Proteins of the Ras superfamily of small GTPases regulate a variety of cellular processes such as intracellular transport, cell shape and motility, as well as differentiation and growth. For all of these processes, switching between the active GTP-bound and the inactive GDP-bound states is of fundamental importance. We describe here the synthesis of reactive acryl derivatives of guanine nucleotides that are able to react covalently with strategically placed cysteines in GTPases to lock them into their functional states in an irreversible manner. Extensive analysis of biochemical and structural features demonstrate the maintenance of the signalling ability of the modified GTPases.

Extending the labelling experiments to other GTPases, placing a cysteine at the position equivalent to E35 in Rab1b led to covalent interaction with aGTP for all those tested (Rab5A, Rab6A, Rab7A, Rab8A, Ypt7, HRas and Cdc42), albeit at variable rates, but substitution of cysteine at positions corresponding to L125 in Rab1b only led to covalent reaction in the case of Rab7A. Using this Ypt7 variant, we were able to produce a covalently linked aGTP adduct that was stable enough to allow crystallization within 12 h at 4 °C and allowed structure determination. In addition to this, we were able to determine the structure of the covalent adduct of the Ypt7Q35C mutant with aGppNHp (for data collection and refinement statistics for Ypt7Q35C–aGDP, Ypt7Q35C–aGppNHp, and Ypt7Q35C, K38I, Q68L–aGTP see Table 1). Structural comparison of these adducts with Ypt7:GDP and Ypt7:GppNHp demonstrates that the covalent linker provides sufficient flexibility to allow the covalently locked proteins to adopt similar conformations of the nucleotide-binding pocket and in particular of the switch I region of Ypt7Q35C–aGDP, Ypt7Q35C–aGppNHp and Ypt7Q35C,K38I,Q68L–aGTP compared with the non-covalently nucleotide-bound proteins. Despite this flexibility, the electron density around the nucleotide and the linker was well defined in Ypt7Q35C–aGDP and Ypt7Q35C,K38I,Q68L–aGTP, whereas in Ypt7Q35C–aGppNHp this was only true for two (chains A and B) out of four copies within the asymmetric unit. In conclusion, the structures of Ypt7 modified with aGDP, aGTP or aGppNHp are very similar to the non-covalent Ypt7:nucleotide complexes, demonstrating that the structural properties of GTPases are maintained in covalently modified proteins.

>[4x]GHMSSRKKNILKVIILGDSGVGKTSLMHRYVNDKYSCQYKATIGADFLTKEVTVDGDKVATMQVWDTAGQERFQSLGVAFYRGADCCVLVYDVTNASSFENIKSWRDEFLVHANVNSPETFPFVILGNKIDAEESKKIVSEKSAQELAKSLGDIPLFLTSAKNAINVDTAFEEIARSALQQNQA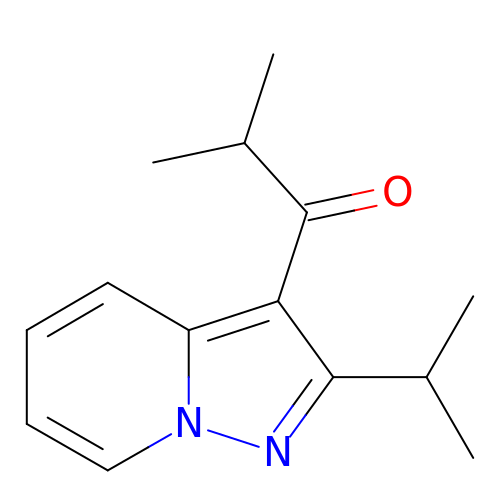2-methyl-1-[2-(propan-2-yl)pyrazolo[1,5-a]pyridin-3-yl]propan-1-one | C14 H18 N2 O | ZJVFLBOZORBYFE-UHFFFAOYSA-N>MGHHHHHHMDYQRINEYLTSIFNNVLVIEEVNLRGSRFKDISIKEMHTIDVIGKAPDVTPSQVSKELMVTLGTVTTSLNNLERKGYIERVRSEQDRRVVHLHLTKKGRLIHRLHKRFHKAMVEKIIDGMSEEEIAV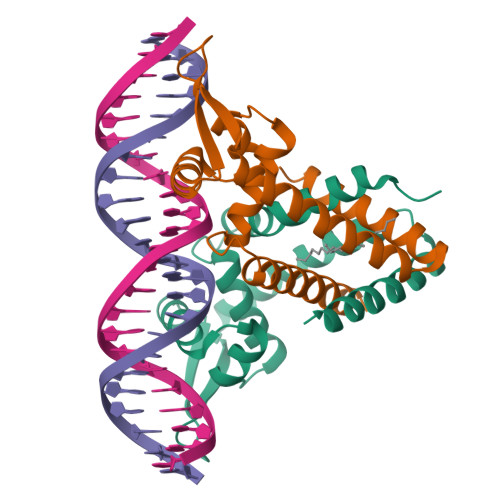MGKGLTNLYQFLEDLK[2x]The polypeptide chain of HlyIIR contains 201 amino acid residues and has a molecular mass of 23.5 kDa. The hemolysin II regulator gene, hlyIIR, is located immediately downstream of hlyII and its product regulates hlyII expression by specifically binding to a 44 bp perfect inverted DNA repeat (22 bp × 2), centred 48 bp upstream of the hlyII transcription initiation point. HlyIIR negatively regulates expression from the hlyII promoter in heterologous system in Escherichia coli cells. In general, the N-terminal domain of HlyIIR exhibits high sequence homology to members of the TetR family while its C-terminal portion appears to be divergent.

In the final model refined at 2.4 Å resolution all residues are within the most favoured and additionally allowed regions of the Ramachandran plot, with all stereochemical values within or better than the expected range. The model contains 179 amino acid residues (Ser4–Lys198) except for a segment of 16 residues (Leu170–Glu185) for which there was no clear electron density. In the crystal structure, the biological dimer is generated by the crystallographic 2-fold axis. The dimer of HlyIIR has an Ω shape, typical for the TetR family of repressors, with overall dimensions of about 60 Å × 60 Å × 25 Å. HlyIIR has an all α-fold, with each subunit consisting of nine α-helices. A monomer of HlyIIR can be subdivided into a small N-terminal DNA-binding domain and a larger C-terminal dimerisation domain. An important feature of the HlyIIR structure is a large internal cavity in the C-terminal α-helical bundle. This cavity is 18 Å long and has an internal volume of ∼ 550 Å3. Most of the inner surface of the cavity is lined by 25 hydrophobic residues contributed by helices α4–α8. The presence of this large cavity and analogy with the structural homologues suggest that DNA-binding properties of HlyIIR are modulated by interactions with a small-molecule ligand.

> MGKSREQTMENILKAAKKKFGERGYEGTSIQEIAKEAKVNVAMASYYFNGKENLYYEVFKKYGLANELPNFLEKNQFNPINALREYLTVFTTHIKENPEIGTLAYEEIIKESARLEKIKPYFIGSFEQLKEILQEGEKQGVFHFFSINHTIHWITSIVLFPKFKKFIDSLGTNETNDTNHEWMPEDLVSRIISALTDKPNI>MEFPIAVHKDDGSVYGVTVPDIPGVHSWGETIDDAIKNTREAIVGHVETLIELGEDVEFTCSTVEELVAKPEYAGA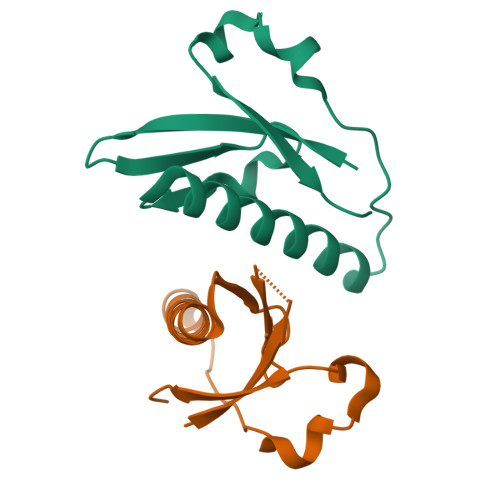VWALVSVDLKHHHHHH[4x]>[6x]MMKRYLLTLAAFAALGALAQSPTLTIYSGRGQSLVEPLVKQFEAE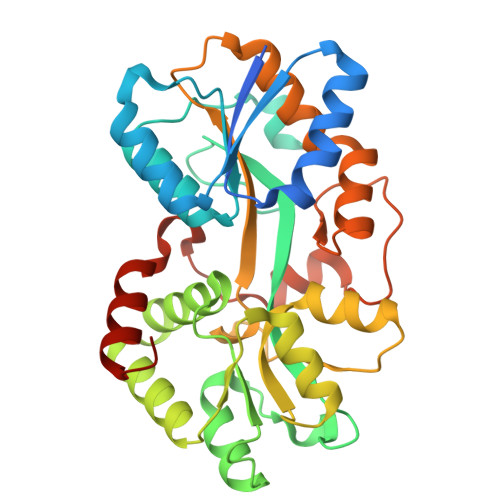TGIRVQVRYSTDAQILAALQEEGSRSPADLFWANTAGALGQASAKGLLRPLGETLLEKPIAFVPASRTWVPVTVRLRVLAYNPDRIKAEELPESLLDLPRFAREKGLVGRVGWTPTYSSFQDMVAGMIALYGEEKTREWLLAMKALAPKAYPSNPAMLDAIRAGEVDLGSTNHYYVVRFRRAGYRLGMHHFRDGDAGNLALVTGAGLLKTSKNLAAATRFLTYLLSPQAQQYFVGNIGEYPLVKGVALDPNLLPLEEALAKSPKLDLEKLPLDRALRLLRETGVLHHHHHH>[2x]MNHFDTIIIGGGPAGMMATISSSFYGQKTLLLEKNKRLGKKLAGTGGGRCNVTNNGNLDDLMAGIPGNGRFLYSVFSQFDNHDIINFFTENGVKLKVEDHGRVFPVTDKSRTIIEALEKKIAELGGTVITNTEIVSVKKTDELFTVRSSDQAWTCQKLIVTTGGKSYPSTG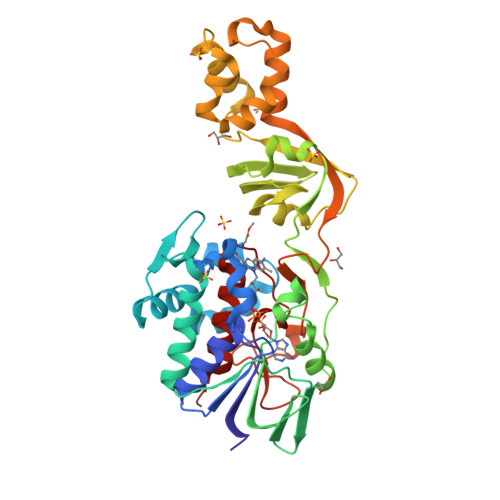STGFGHDIARHFKHTVTDLEAAESPLLTDFPHKALQGISLDDVTLSYGKHIITHDLLFTHFGLSGPAALRLSSFVKGGETIYLDVLPQMSQQDLADFLEEHREKSLKNCLKILLPERIADFFTQPFPEKVKQLNLSEKEALIKQIKELPISVTGKMSLAKSFVTKGGVSLKEINPKTLESKLVPGLHFAGEVLDINAHTGGFNITSALCTGWVAGSLHYD5-azanyl-3-[1-[[4-(morpholin-4-ylmethyl)phenyl]methyl]indol-6-yl]-1~{H}-pyrazole-4-carbonitrile | C24 H24 N6 O | 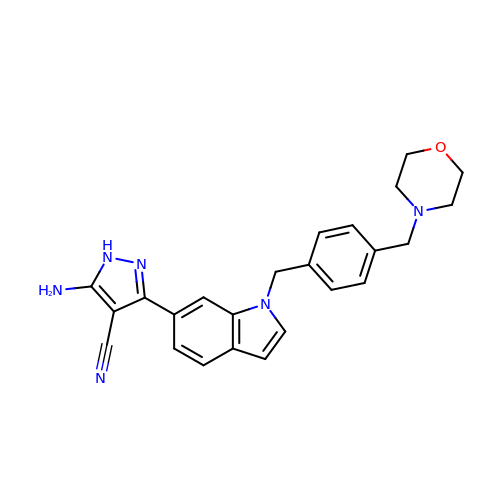UYOMCTXSEJZTSM-UHFFFAOYSA-N> GAMGSKICQFKLVLLGESAVGKSSLVLRFVKGQFHEYQESTIGAAFLTQTVCLDDTTVKFEIWDTAGLERYHSLAPMYYRGAQAAIVVYDITNTDTFARAKNWVKELQRQASPNIVIALAGNKADLASKRAVEFQEAQAYADDNSLLFMETSAKTA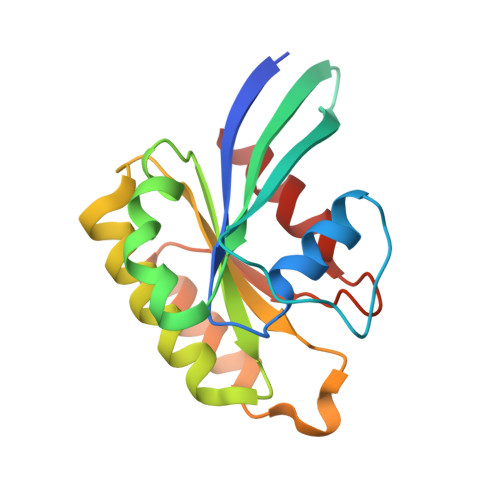MNVNEIFMAIAKKL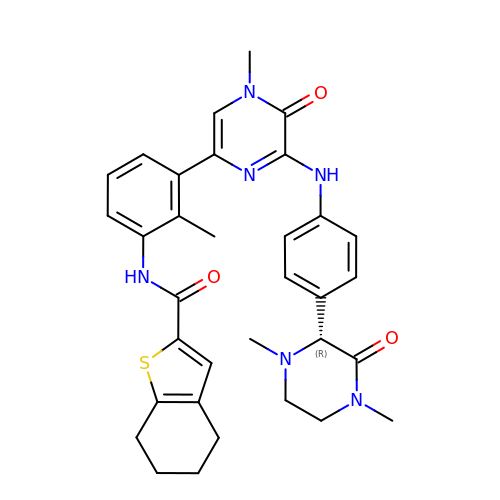N-{3-[6-({4-[(2R)-1,4-dimethyl-3-oxopiperazin-2-yl]phenyl}amino)-4-methyl-5-oxo-4,5-dihydropyrazin-2-yl]-2-methylphenyl}-4,5,6,7-tetrahydro-1-benzothiophene-2-carboxamide | C33 H36 N6 O3 S | CDOOFZZILLRUQH-GDLZYMKVSA-N>MAEQVKPAGVKPKGTVPPPKGNAPAPKANGAPGGASVIKEQDAAKMRRFLFQRTETRSTKWYQIFDTEKLDDEQVVGGHLALLGVLGFIMGIYYISGIQVFPWGAPGFHDNWFYLTIKPRMVSLGIDTYSTKTADLEAAGARLLGWAAFHFLVGSVLIFGGWRHWTHNLTNPFTGRCGNFRDFRFLGKFGDVVFNGTSAKSYKEALGPHAVYMSLLFLGWGIVMWAILGFAPIPDFQTINSETFMSFVFAVIFFALGIYWWNNPPNAAIHLNDDMKAAFSVHLTAIGYINIALGCIAFVAFQQPSFAPYYKELDKLVFYLYGEPFNRVSFNFVEQGGKVISGAKEFADFPAYAILPKSGEAFGMARVVTNLIVFNHIICGVLYVFAGVYHGGQYLLKIQLNGMYNQIKSIWITKGRDQEVQVKILGTVMALCFATMLSVYAVIVWNTICELNIFGTNITMSFYWLKPLPIFQWMFADPSINDWVMAHVITAGSLFSLIALVRIAFFAHTSPLWDDLGLKKNSYSFPCLGPVYGGTCGVSIQDQLWFAMLWGIKGLSAVCWYIDGAWIASMMYGVPAADAKAWDSIAHLHHHYTSGIFYYFWTETVTIFSSSHLSTILMIGHLVWFISFAVWFEDRGSRLEGADIQTRTIRWLGKKFLNRDVNFRFPVLTISDSKLAGTFLYFGGTFMLVFLFLANGFYQTNSPLPPPVSHAAVSGQQMLAQLVDTLMKMIA[2x];> MAEPVENKNQAPAPGAKVPPKGAPAAPKAGAPAAPKGPVAPKAGAPAAKTGASAAKQAGKPRLASLGVTLGRSGVRQESALPYVKPKAVPPPKPAAPAAKGAPAPKGAPAAPAAKAAPGAPVAKAAPKAKKHYFIIENLCVGCGLCLDKCPPKVNAIGYKFYGDVQEGGFRCYIDQAACISCSACFSGDECPSGALIEVLPDGEVLDFSYTPPERLDFDLRFLHRFHREAR;>MDKNSNGKLIALAVGGAVLMGALFFSVSFLTGYIPAPNHSAILTPLRSFMGWFLLIFCASIIIMGLGKMSSAISDKWFLSFPLSIFVIVMVMFLSLRVYWEKGRTTTVDGKYIRTTAELKEFLNKPAATSDVPPAPAGFDFDAAKKLVDVRCNKCHTLDSVADLFRTKYKKTGQVNLIVKRMQGFPGSGISDDDAKTIGIWLHEKF[2x];> MQPQLSRPQTASNQVRKAVSGPWSGNAVHKAEKYFITSAKRDRDGKLQIELVPASGRRKLSPTPEMIRRLIDGEIEIYILTTQPDIAIDMNKEIIDMENRYVIDFDKRGVKWTMREIPVFYHEGKGLCVELHNKIYTLDQFFK;>MALFGSNDVTTAHSDYEIVLEGGSSSWGKVKARAKVNAPPASPLLPADCDVKLNVKPLDPAKGFVRISAVFESIVDSTKNKLTIEADIANETKERRISVGEGMVSVGDFSHTFSFEGSVVNLFYYRSDAVRRNVPNPIYMQGRQFHDILMKVPLDNNDLIDTWEGTVKAIGSTGAFNDWIRDFWFIGPA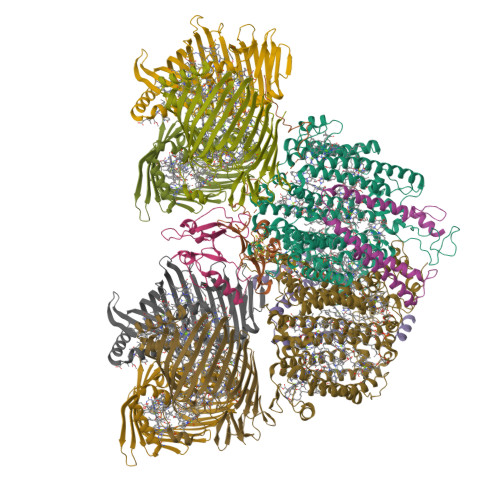FTALNEGGQRISRIEVNGLNTESGPKGPVGVSRWRFSHGGSGMVDSISRWAELFPSDKLNRPAQVEAGFRSDSQGIEVKVDGEFPGVSVDAGGGLRRILNHPLIPLVHHGMVGKFNNFNVDAQLKVVLPKGYKIRYAAPQYRSQNLEEYRWSGGAYARWVEHVCKGGVGQFEILYAQ[6x]> MQQASTPTIGMIVPPAAGLVPADGARLYPDLPFIASGLGLGSVTPEGYDAVIESVVDHAR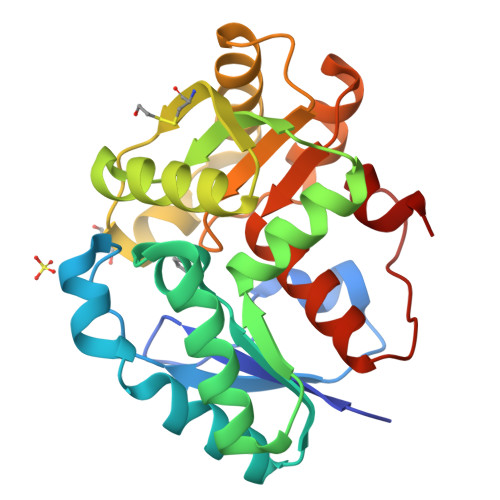RLQKQGAAVVSLMCTSLSFYRGAAFNAALTVAMREATGLPCTTMSTAVLNGLRALGVRRVALATAYIDDVNERLAAFLAEESLVPTGCRSLGITGVEAMARVDTATLVDLCVRAFEAAPDSDGILLSSGGLLTLDAIPEVERRLGVPVVSSSPAGFWDAVRLAGGGAKARPGYGRLFDES>[2x]STTEVVMENVTAFWEEGFGELFEKAKQNNNNRKTSNGDDSLFFSNFSLLGTPVLKDINFKIERGQLLAVAGSTGAGKTSLLMMIMGELEPSEGKIKHSGRISFCSQNSWIMPGTIKENIIGVSYDEYRYRSVIKACQLEEDISKFAEKDNIVLGEGGITLSGGQRARISLARAVYKDADLYLLDSPFGYLDVLTEKEIFESCVCKLMANKTRILVTSKMEHLKKADKILILHEGSSYFYG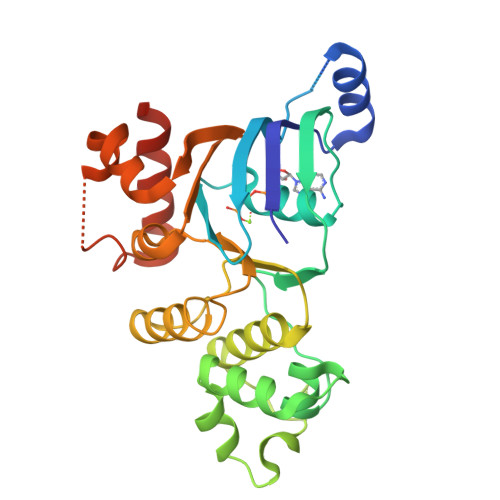TFSELQNLRPDFSSKLMGCDSFDQFSAERRNSILTETLHRFSLEGDAPVS>[2x]MGSSHHHHHHSSGLVPRGSKKKKEMPFPNKKIELGDKLSESIRSFSTITDTEIIIGICRKNIPGWKEINESYIEVKQIFSGLTNQLFVVSIVNESMSLSLKHPRILFRIYGKHVGKFYDSKVELDVFRYLSNINIAPNIIADFPEGRIEEFIDGEPLTTKQLQLTHICVEVAKNMG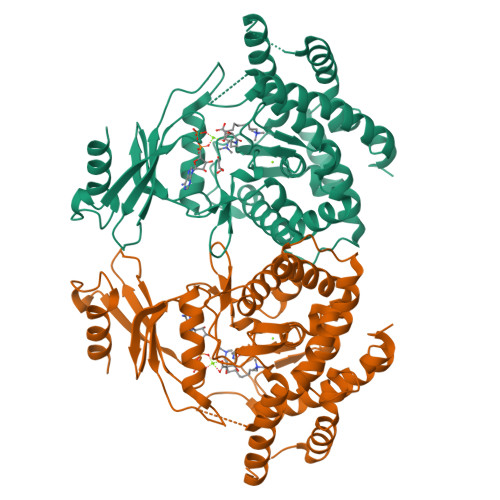SLHIINSKRADFPSRFDKEPILFKRIYLWREEAKIQVSKNNFQIDKELYSKILEEIDQLEELIMGGEKFSMERALELKLYSPAFSLVFAHNDLQENNLLQTQNNIRMIDYEYSAINFAGADIANYFCEYIYDYCSEKQPYFKFKYEDYPCEELRKLFISVYLSQTLQEQVMPSQQIVHIMTKAVEVFTLISHITWGLWSIARTPGYQPNSVEFDFTEYANTRFTHYLQKKKELIDQGILPLNSWLFNL> GAMDRLRAAEHPRPDYVLLHISDTHLIGGDRRLYGAVDADDRLGELLEQLNQSGLR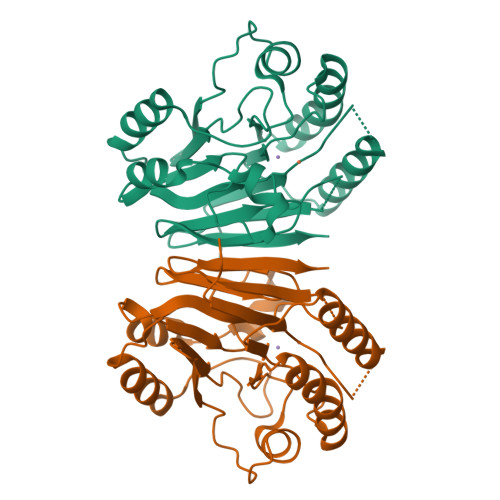PDAIVFTGDLADKGEPAAYRKLRGLVEPFAAQLGAELVWVMGAHDDRAELRKFLLDEAPSMAPLDRVCMIDGLRIIVLDTSVPGHHHGEIRASQLGWLAEELATPAPDGTILALHHPPIPSVLDMAVTVELRDQAALGRVLRGTDVRAILAGHLHYSTNATFVGIPVSVASATCYTQDLTVAAGGTRGRDGAQGCNLVHVYPDTVVHSVIPLGGGETVGTFVSP>KDWTQYVNPLMGSQSTFELSTGNTYPAIARPWGMNFWTPQTGKMGDGWQYTYTANKIRGFKQTHQPSPWINDYGQFSIMPIVGQPVFDEEKRASWFAHKGEVATPYYYKVYLAEHDIVTEMTPTERAVLFRFTFPENDHSYVVVDAFDKGSYIKIIPEENKIIGYTTRNSGGVPENFKNYFIIEFDKPFTYKATVENGNLQENVAEQTTDHAGAIIGFKTRKGEQVNARIASSFISFEQAAANMNELGKDNIEQLAQKGKDAWNQVLGKIEVEGGNLDQYRTFYSCLYRSLLFPRKFYELDANGQPIHYSPYNGQVLPGYMFTDTGFWDTFRCLFPLLNLMYPSVNKEMQEGLINTYLESGFFPEWASPGHRGCMVGNNSASILVDAYMKGVKVDDIKTLYEGLIHGTENVHPEVSSTGRLGYEYYNKLGYVPYDVKINENAARTLEYAYDDWCIYRLAKELKRPKKEISLFAKRAMNYKNLFDKESKLMRGRNEDGTFQ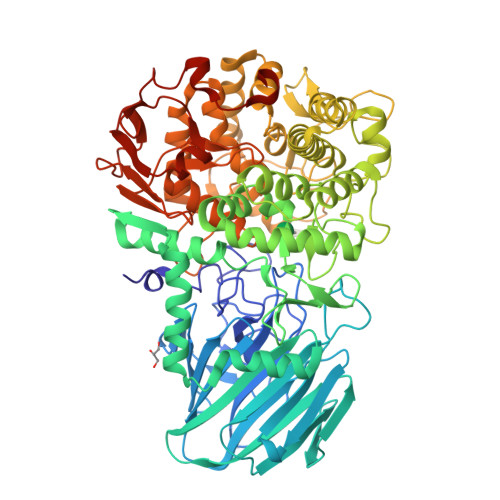SPFSPLKWGDAFTEGNSWHYTWSVFHDPQGLIDLMGGKEMFVTMMDSVFAVPPIFDDSYYGQVIHEIREMTVMNMGNYAHGNQPIQHMIYLYDYAGQPWKAQYWLRQVMDRMYTPGPDGYCGDEDNGQTSAWYVFSALGFYPVCPGTDEYVMGTPLFKKATLHFENGNSLVIDAPNNSTENFYIDSMSFNGADHTKNYLRHEDLFKGGTIKVDMSNRPNLNRGTKEEDMPYSFSKELEHHHHHH[6x]>MAHHHHHHVGTGSNDDDDKSPDPNWELVYTARLQEFMFTFIPITHPTSDTKHPLLLVQSAHGEKYFFGKIGEGSQRSLTENKIRISKLKDIFLTGELNWSDIGGLPGMILTIADQGKSNLVLHYGNDILNYIVSTWRYFVFRFGIDLNDHIMKDKEVYKDKIIAVKSFNVLKNGGEDRLGVFDSFQKGVLRSIVAKMFPKHAPTDRYDPSSDPHLNVELPDLDAKVEVSTNYEISFSPVRGKFKVEEAIKLGVPKGPLFAKLTKGQTITLDNGIVVTPEQVLENERHFAKVLILDIPDDLYLNAFVEKFKD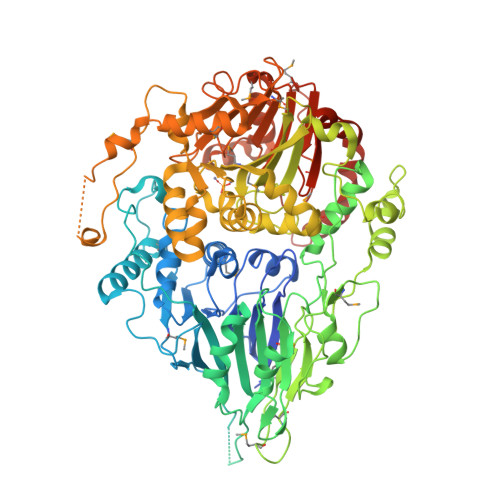YDCAELGMVYYFLGDEVTINDNLFAFIDIFEKNNYGKVNHMISHNKISPNTISFFGSALTTLKLKALQVNNYNLPKTDRVFSKDFYDRFDTPLSRGTSMCKSQEEPLNTIIEKDNIHIFSQNKTVTFEPFRMNEEPMKCNINGEVADFSWQEIFEEHVKPLEFPLADVDTVINNQLHVDNFNNSAEKKKHVEIITLGTGSALPSKYRNVVSTLVKVPFTDADGNTINRNIMLDAGENTLGTIHRMFSQLAVKSIFQDLKMIYLSHLHADHHLGIISVLNEWYKYNKDDETSYIYVVTPWQYHKFVNEWLVLENKEILKRIKYISCEHFINDSFVRMQTQSVPLAEFNEILKENSNQESNRKLELDRDSSYRDVDLIRQMYEDLSIEYFQTCRAIHCDWAYSNSITFRMDENNEHNTFKVSYSGDTRPNIEKFSLEIGYNSDLLIHEATLENQLLEDAVKKKHCTINEAIGVSNKMNARKLILTHFSQRYPKLPQLDNNIDVMAREFCFAFDSMIVDYEKIGEQQRIFPLLNKAFVEEKEEEEDVDDVESVQDLEVKLKKHKKN[2x]>MPRGLELLIAQTILQGFDAQYGRFLEVTSGAQQRFEQADWHAVQQAMKNRIHLYDHHVGLVVEQLRCITNGQSTDAEFLLRVKEHYTRLLPDYPRFEIAESFFNSVYCRLFDHRSLTPERLFIFSSQ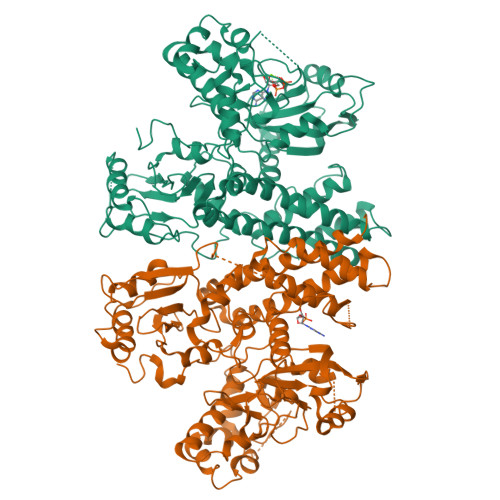PERRFRTIPRPLAKDFHPDHGWESLLMRVISDLPLRLHWQNKSRDIHYIIRHLTETLGPENLSKSHLQVANELFYRNKAAWLVGKLITPSGTLPFLLPIHQTDDGELFIDTCLTTTAEASIVFGFARSYFMVYAPLPAALVEWLREILPGKTTAELYMAIGCQKHAKTESYREYLVYLQGCNEQFIEAPGIRGMVMLVFTLPGFDRVFKVIKDKFAPQKEMSAAHVRACYQLVKEHDRVGRMADTQEFENFVLEKRHISPALMELLLQEAAEKITDLGEQIVIRHLYIERRMVPLNIWLEQVEGQQLRDAIEEYGNAIRQLAAANIFPGDMLFKNFGVTRHGRVVFYDYDEICYMTEVNFRDIPPPRYPEDELASEPWYSVSPGDVFPEEFRHWLCADPRIGPLFEEMHADLFRADYWRALQNRIREGHVEDVYAYRRRQRFSVRYGEMLF[2x]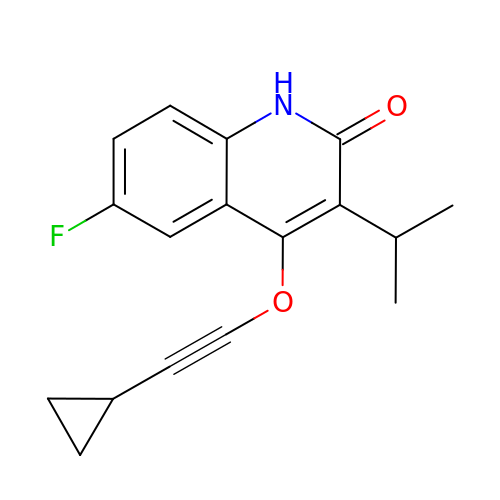4-[(CYCLOPROPYLETHYNYL)OXY]-6-FLUORO-3-ISOPROPYLQUINOLIN-2(1H)-ONE | C17 H16 F N O2 | YVJFHKQYMKKIHK-UHFFFAOYSA-N> MGIPILKLGECLLISIQSELDDHTAVEFQEDLLAKIHETSARGVVIDITSIDFIDSFIAKILGDVVSMSKLMGAKVVVTGIQPAVAITLIELGITFSGVLSAMDLE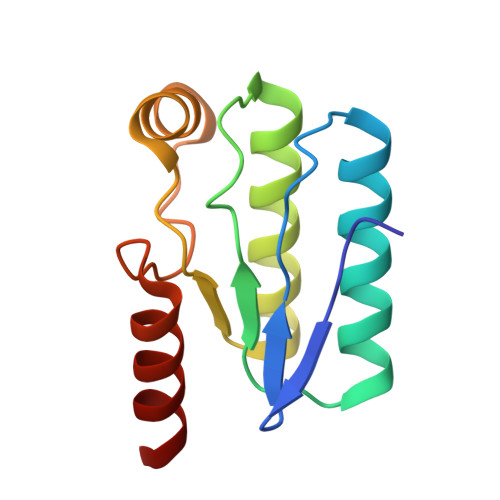SGLEKLKQELGE>[2x]MRLCDRDIEAWLDEGRLSINPRPPVERINGATVDVRLGNKFRTFRGHTAAFIDLSGPKDEVSAALDRVMSDEIVLDEGEAFYLHPGELALAVTLESVTLPADLVGWLD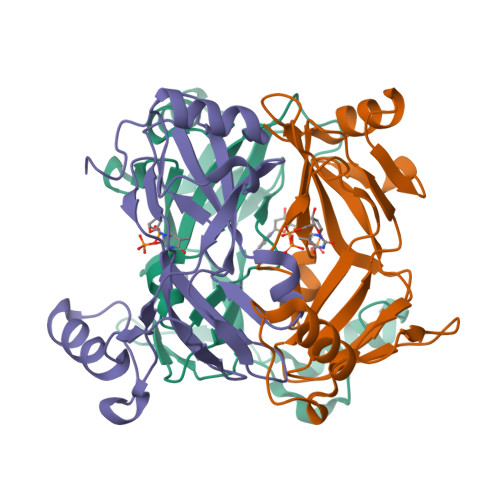GRSSLARLGLMVHVTAHRIDPGWSGCIVLAFYNSGKLPLALRPGMLIGALSFEPLSGPAVRPYNRREDAKYRNQQGAVASRIDKD>GDYDLVVVGGGIVGAASAREIVLRHPSLKVAVLEKECKLAKHQSGHNSGVIHAGIYYKPGTLKARLCVEGMHLAYAYLDEKKIPYKKTGKLIVATDEKEVKLLKDLEKRGIANNVPDLRMIEGSEIQEIEPYCQGVMALHSPHTGIVDWGLVTEHYGQDFKQCGGDIYLDFNVSKFTETKEGTDYPVTIHGAKPGQTVRTKNVLTCGGLQSDLLAEKTGCPRDPRIVPFRGEYLLLTKEKQHMVKGNIYPVPDPRFPFLGVHFTPRMDGSIWLGPNAVLALKREGYTWGDINLFELFDALRYPGFVKMASKYIGFGLSEMSKSWFINLQIKALQKYIPDITEYDIQRGPAGVRAQAMDLDGNLVDDFVFDRGQGSGALAKRVLHCRNAPSPGATSSLAIAKMIADKIENEFSIGK[4x]

l-2-hydroxyglutarate dehydrogenase (L2HGDH) is a mitochondrial membrane–associated metabolic enzyme, which catalyzes the oxidation of l-2-hydroxyglutarate (l-2-HG) to 2-oxoglutarate (2-OG). L2HGDH belongs to the d-amino acid oxidase (DAAO) family of the FAD-dependent proteins. Like other members of the DAAO family, dmL2HGDH is composed of the FAD-binding domain and the substrate-binding domain. The active site of dmL2HGDH is located at the interface of the FAD-binding domain and the substrate-binding domain and is composed of residues from both domains.

Crystallization of dmL2HGDH in the absence of any ligands yielded crystals in FAD-bound form (dmL2HGDHFAD) and in complex with FAD and SO42− (dmL2HGDHFAD+SO4) in which SO42− was derived from the crystallization solution. Structures of dmL2HGDH in FAD-bound form and in complex with FAD and SO42− or 2-OG were determined at resolutions of 2.85 Å, 2.30 Å, and 2.82 Å, respectively. In the dmL2HGDHFAD+SO4 structure, there is a SO42− anion bound at the substrate-binding site, which occupies a similar position as the C1-carboxyl of 2-OG and makes similar interactions with the surrounding residues except for Leu299. In all structures, there are four dmL2HGDH monomers forming a tetramer in the asymmetric unit. In each monomer, there are an FAD bound at the active site and a detergent molecule n-dodecyl-β-d-maltopyranoside (DDM) on a surface groove. The DDM molecule is derived from the purification buffer with its hydrophilic head lying on the protein surface and the hydrophobic tail pointing to the interior of the protein, which might stabilize the structure. In all structures, an FAD molecule is bound at the FAD-binding site, which adopts an elongated conformation with the isoalloxazine moiety pointing toward the substrate-binding site and forming extensive hydrophilic and hydrophobic interactions with the surrounding residues.>MSKKEVCSVAFLKAVFAEFLATLIFVFFGLGSALKWPSALPTILQIALAFGLAIGTLAQALGPVSGGHINPAITLALLVGNQISLLRAFFYVAAQLVGAIAGAGILYGVAPLNARGNLAVNALNNNTTQGQAMVVELILTFQLALCIFASTDSRRTSPVGSPALSIGLSVTLGHLVGIYFT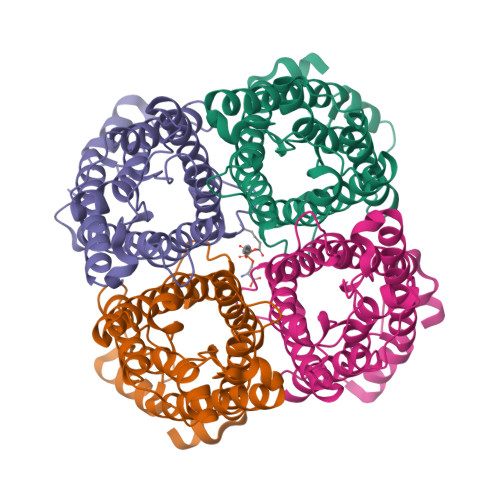GCSMNPARSFGPAVVMNRFSPAHWVFWVGPIVGAVLAAILYFYLLFPNSLSLSERVAIIKGTYEPDEDWEEQREERKKTMELTTR[4x]>GSVHTSPKVKNLNPKKFSIHDQDHKVLVLDSGNLIAVPDKNYIRPEIFFALASSLSSASAEKGSPILLGVSKGEFCLYCDKDKGQSHPSLQLKKEKLMKLAAQKESARRPFIFYRAQVGSWNML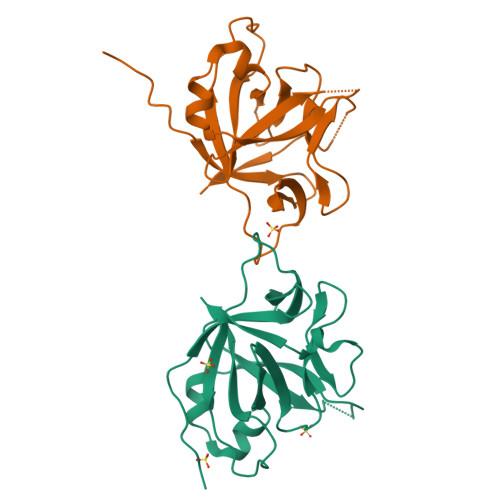ESAAHPGWFICTSCNCNEPVGVTDKFENRKHIEFSFQPVCKAEMSPSEVSD[2x]> MSRWLWPWSNCVKERVCRYLLHHYLGHFFQEHLSLDQLSLDLYKGSVALRDIHLEIWSVNEVLESMESPLELVEGFVGSIEVAVPWAALLTDHCTVRVSGLQLTLQPRRGPAPGAADSQSWASCMTTSLQLAQECLRDGLPEPSEPPQPLEGLEMFAQTIETVLRRIKVTFLDTVVRVEHSPGDGERGVAVEVRVQRLEYCDEAVRDPSQAPPV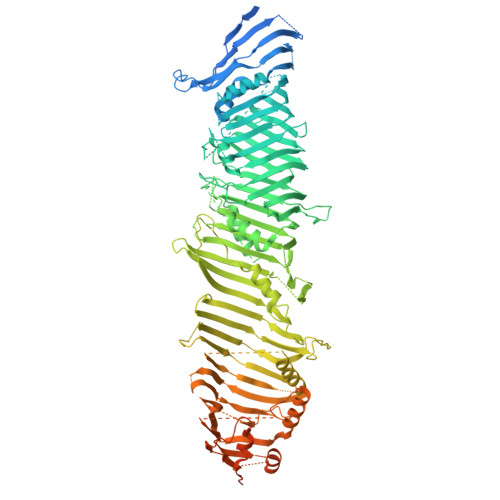DVHQPPAFLHKLLQLAGVRLHYEELPAQEEPPEPPLQIGSCSGYMELMVKLKQNEAFPGPKLEVAGQLGSLHLLLTPRQLQQLQELLSAVSLTDHEGLADKLNKSRPLGAEDLWLIEQDLNQQLQAGAVAEPLSPDPLTNPLLNLDNTDLFFSMAGLTSSVASALSELSLSDVDLASSVRSDMASRRLSAQAHPAGKMAPNPLLDTMRPDSLLKMTLGGVTLTLLQTSAPSSGPPDLATHFFTEFDATKDGPFGSRDFHHLRPRFQRACPCSHVRLTGTAVQLSWELRTGSRGRRTTSMEVHFGQLEVLECLWPRGTSEPEYTEILTFPGTLGSQASARPCAHLRHTQILRRVPKSRPRRSVACHCHSELALDLANFQADVELGALDRLAALLRLATVPAEPPAGLLTEPLPAMEQQTVFRLSAPRATLRLRFPIADLRPEPDPWAGQAVRAEQLRLELSEPQFRSELSSGPGPPVPTHLELTCSDLHGIYEDGGKPPVPCLRVSKALDPKSTGRKYFLPQVVVTVNPQSSSTQWEVAPEKGEELELSVESPCELREPEPSPFSSKRTMYETEEMVIPGDPEEMRTFQSRTLALSRCSLEVILPSVHIFLPSKEVYESIYNRINNDLLMWEPADLLPTPDPAAQPSGFPGPSGFWHDSFKMCKSAFKLANCFDLTPDSDSDDEDAHFFSVGASGGPQAAAPEAPSLHLQSTFSTLVTVLKGRITALCETKDEGGKRLEAVHGELVLDMEHGTLFSVSQYCGQPGLGYFCLEAEKATLYHRAAVDDYPLPSHLDLPSFAPPAQLAPTIYPSEEGVTERGASGRKGQGRGPHMLSTAVRIHLDPHKNVKEFLVTLRLHKATLRHYMALPEQSWHSQLLEFLDVLDDPVLGYLPPTVITILHTHLFSCSVDYRPLYLPVRVLITAETFTLSSNIIMDTSTFLLRFILDDSALYLSDKCEVETLDLRRDYVCVLDVDLLELVIKTWKGSTEGKLSQPLFELRCSNNVVHVHSCADSCALLVNLLQYVMSTGDLHPPPRPPSPTEIAGQKLSESPASLPSCPPVETALINQRDLADALLDTERSLRELAQPSGGHLPQASPISVYLFPGERSGAPPPSPPVGGPAGSLGSCSEEKEDEREEEGDGDTLDSDEFCILDAPGLGIPPRDGEPVVTQLHPGPIVVRDGYFSRPIGSTDLLRAPAHFPVPSTRVVLREVSLVWHLYGGRDFGPHPGHRARTGLSGPRSSPSRCSGPNRPQNSWRTQGGSGRQHHVLMEIQLSKVSFQHEVYPAEPATGPAAPSQELEERPLSRQVFIVQELEVRDRLASSQINKFLYLHTSERMPRRAHSNMLTIKALHVAPTTNLGGPECCLRVSLMPLRLNVDQDALFFLKDFFTSLVAGINPVVPGETSAEARPETRAQPSSPLEGQAEGVETTGSQEAPGGGHSPSPPDQQPIYFREFRFTSEVPIWLDYHGKHVTMDQVGTFAGLLIGLAQLNCSELKLKRLCCRHGLLGVDKVLGYALNEWLQDIRKNQLPGLLGGVGPMHSVVQLFQGFRDLLWLPIEQYRKDGRLMRGLQRGAASFGSSTASAALELSNRLVQAIQATAETVYDILSPAAPVSRSLQDKRSARRLRRGQQPADLREGVAKAYDTVREGILDTAQTICDVASRGHEQKGLTGAVGGVIRQLPPTVVKPLILATEATSSLLGGMRNQIVPDAHKDHALKWRSDSAQD> MIDQKIFETTLNIDDPTNFCTNVEAHLLKELENIYVGKCFKNSFILNITGVIQRSPCFIMRTNNSGRGYMHVRFSAVVSYLNAFDLIAAVKIIKNDSNIILGESLLTEPVTIVIPSSESQNNVAEVGQIVPVQLANSSVYYIPGRQQASATGSIFIPKHTFSVYHVQEELTQEQALNLTKLVNIIEMLLESRSKKDFKQICFFEKLYYTYSISSDEILDLKIWKGPKGKEMSRLKPCNVLSFLYDALKNKNSSLGFWARPPNLL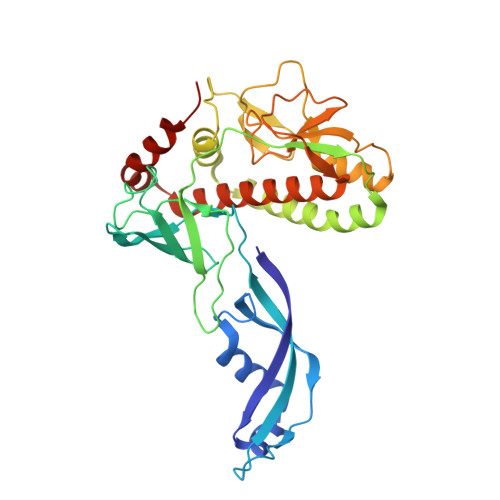KSSPLAYQQDQNSFNATELPIICSAEVMFVTLLKEIINYLQFINDLCDTFNNEQLIKRHENIWMLIEQRKIGHDF>VAVEEFPRKLLTFKEKLGEGQFGEVHLCEVEGMEKFKDKDFALDVSANQPVLVAVKMLRADANKNARNDFLKEIKIMSRLKDPNIIHLLAVCITDDPLCMITEYMENGDLNQFLSRHEPPNSSSSDVRTVSYTN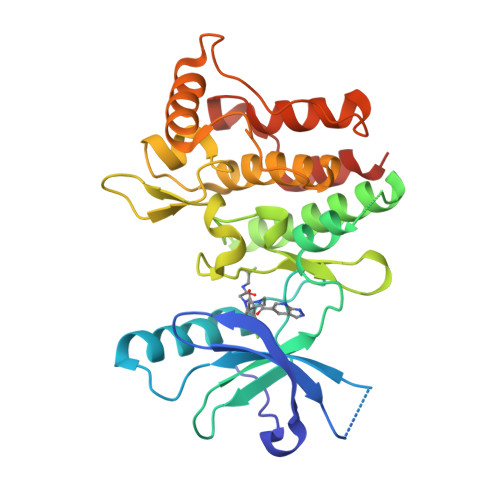LKFMATQIASGMKYLSSLNFVHRDLATRNCLVGKNYTIKIADFGMSRNLYSGDYYRIQGRAVLPIRWMSWESILLGKFTTASDVWAFGVTLWETFTFCQEQPYSQLSDEQVIENTGEFFRDQGRQTYLPQPAICPDSVYKLMLSCWRRDTKNRPSFQEIHLLLLQQGDEHHHHHH[12x]>GSMLDGPYQPTTFTPPSDYWILINSNTNGVVYESTNNSDFWTAVIAVEPHVDPVDRQYNVFGENKQFNVRNDSDKWKFLEMF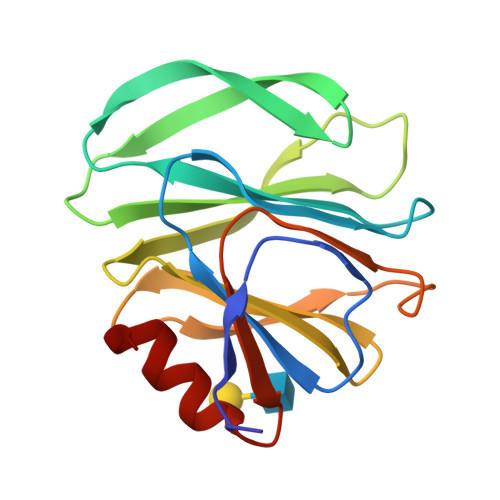RGSSQNDFYNRRTLTSNTRLVGILKYGGRIWTFHGETPRATTDSSNTANLNGISITIHSEFYIIPRSQESKCNEYINNGL[2x]>[2x]GNEEETNNYTPVDNQSNSTSEIILQERNSSLPRVWSKKTAQRVTTRASFTDATDFLGCSYAVENGTSIIGDFANAKYPVVNMKKLLERYPSYINPKELRTTETKALSYSDFDRLEKNKTFTKTVKSGFSLNLGPFKFGRQKTIKETFVHNTDDSEKVVHGELSIEVVNGMLNLQTAPSALRKIAADYLDELFVDALYNSSMVELMQSYGEFVLTGYYTGGRASALFYGVDTNSIQFDSKEKDMDVAINASYEWKNKKPTAPSDTIHSASGNLSIGTKRE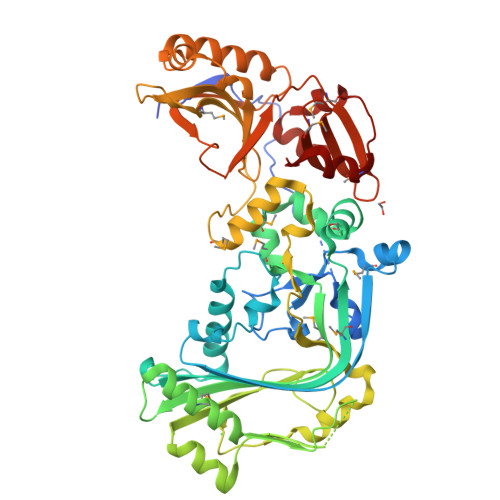NSETITNKFSALSYSIKTLGGAYGYSISTPPYDITNYSIDLTPWLQSLNDPKTHTMIDLQDGGLYPISDFILEENFKQRYNDTHMDFQYQESLEEPYIEIIKMYIRKSNSGEKLYDIVPVLNTRQGDKLIFSNPDAASQSDEELKANSIPATFLTKSNAIKDEKSKYYQLKIKADPNKTINPIIQTTLSFQINNVDEKGMYKFKNANTNIWYIYNPTSMYCFAYYDDDYIPDAYGILDWVNGIPIKAVTMTTLYQRYKIYGL>[2x]MGSSHHHHHHSSGLVPRGSTYKLTLIRHGESEWNKENRFTGWTDVSLSEQGVSEAIEAGRMLLEKGFKFDVVYTSVLKRAIMTTWTVLKELGNINCPIINHWRLNERHYGALQGLNKSETASKFGEDQVKIWRRSFDVPPPVLEKSDPRWPGNELIYKGICPSCLPTTECLKDTVERVKPYFEDVIAPSIMSGKSVLVSAHGNSLRALLYLLEGMTPEQILEVNIPTACPL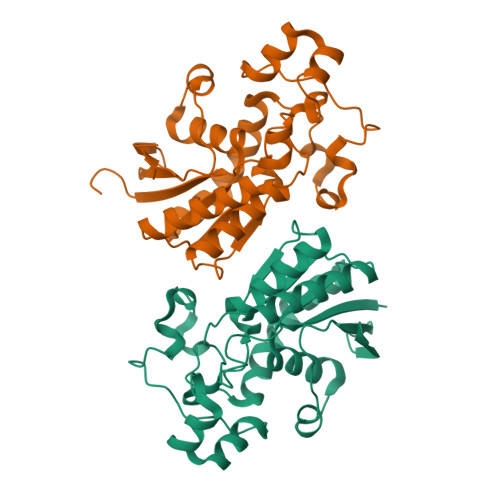VLELDDYLKVTKKYYLISEEELKAKMEAVANQGKAK>HDDRRTLWTTPDPSPNCTIDEERDSKLTLVLTKCGSQILANVSLLVVKGKFSNINNNTNPTDKKITVKLLFNEKGVLMDSSSLKKEYWNYRNDNSTVSQAYDNAVPFMPNIKAYPKPTTDTSAKPEDKKSAAKRYIVSNVYIGGLPDKTVVITIKLNAETESAYSMTFEFTWAKTFENLQFDSSSFTFSYIAQEN[3x]

Each protein forms key interactions to promote cell infection, with the terminal domain of the fiber, the fiber knob protein, interacting with the viruses’ primary cell entry receptor. The adenovirus fiber knob protein is known to have a highly conserved trimeric structure. Sialic acid (SA) usage has been proposed as a cell infection mechanism for EKC causing HAdV-D. Here we highlight an important role for SA engagement by many HAdV-D. We provide apo state crystal structures of 7 previously undetermined HAdV-D fiber-knob proteins, and structures of HAdV-D25, D29, D30 and D53 fiber-knob proteins in complex with SA. Our findings demonstrate a conserved binding site for sialic acid, common across the species D adenoviruses, therefore suggesting that, along with CAR, the receptor can be used to initiate cell entry.

We performed X-ray crystallography to generate structures of species D human adenovirus fiber knob proteins HAdV-D15, D24, D29, D30, D32 and D53 in their apo states. HAdV-D15, D24 and D32 were crystallised in only their apo states, whereas HAdV-D25, D29, D30 and D53 crystals were also soaked with sialic acid. Additionally, crystals of HAdV-D32 fiber knob protein soaked with sialic acid could not be obtained. CAR binding was investigated for fiber knob proteins of HAdV-D24, D26 and D32, and was found to be significantly weaker interacting. The respective IC50 values were quantified as 0.02931, 0.001261 and 0.01996 µg/10e5 cells. These values represent fold changes of 162, 6 and 110 times weaker compared with the IC50 value measured for HAdV-C5 fiber knob protein.> MHRVMGIETEYGISVPHQPNANAMAASSQVVNAYAPIGAPAQRQARWDFEEENPLRDARGFEVAREAADPSQLTDEDLGLANVILTNGARLYVDHAHPEYSTPEVTNPRDAVLWDKAGERIMAEAARRAADLPMGWTIQLYKNNTDNKGASYGCHENYLMNRSTPFADIVRHLIPFFVTRQVFCGAGRVGIGADGRGEGFQLSQRADFFEVEVGLETTLKRPIINTRDEPHADPEKYRRLHVIIGDANMSEIATYLKLGTTALVLAMIEDGFLSQDFSVESPVGALRAVSHDPTLRYQLRLHDGRRLTAVQLQMEYLEQARKYVEDRFGTDVDDMTRDVLDRWETTLVRLADDPMQLSRDLDWVAKLSILEGYRQRENLPWSAHKLQLVDLQYHDVRPDRGLYNRLVARGRMNLLVDEAAVRTAMHEPPNDTRAYFRGRCLAKFGAEIAAASWDSVIFDLPGRDSLQRVPTLEPLRGTRAHVGDLLDRCRSATELVAALTGGENLYFQ

Pupylation is the post-translational modification of lysine side chains with prokaryotic ubiquitin-like protein (Pup) that targets proteins for proteasomal degradation in mycobacteria and other members of Actinobacteria. A single Pup ligase enzyme, PafA (proteasome accessory factor A), is responsible for modifying all pupylation substrate proteins and likewise a single depupylase enzyme, Dop (deamidase of Pup), removes Pup from Pup-protein adducts. Depupylase Dop is structurally homologous to Pup ligase PafA, although the two evolutionarily related enzymes catalyze opposing reactions. Rather, before the catalytic cycle of Dop can begin, Dop-mediated cleavage of ATP in the active site must take place to generate the Pi species important for catalysis.

With the aim to capture Dop in a state where the Dop-loop could be resolved, crystallization experiments were carried out with AcelDop, exploring conditions with Dop alone and Dop in complex with Pup and/or different adenine nucleotides. We were successful in identifying crystallization conditions, where AcelDop in the absence of other ligands features the Dop-loop in a well-resolved conformation that is not induced via crystal contacts. In this structure, 33 of the 40 residues in the Dop-loop are resolved, including residues P40–R65 and L73–L80 and thereby all of the highly conserved residues in the loop. The Dop-loop features two very short helical stretches (DLη1 and DLα1) flanking a long zigzagging loop. Helix DLη1 (η stands for 310 helix) consists of residues 48-52 (DFEEE) and is located nearby the nucleotide-binding pocket (NBP) of Dop, while DLα1 is formed by residues 75-78 (DEDL) and is positioned distal to the active site. The Dop-loop forms extensive interactions with residues surrounding the active site. In particular, insertion of the highly conserved Dop-loop-residue W47 into the NBP leads to the formation of a triple π-stack, where W47 interacts with H231 that in turn stacks with W453 of the C-terminal domain. Another π-stacking interaction is formed by Dop-loop-residue F49 and H155. Furthermore, a network of salt bridges is formed between acidic residues in the Dop-loop and several arginine side chains surrounding the active site. Superimposition of the Dop-loop-inserted structure with any of the Pup-bound structures reveals dramatic conformational changes of the Dop-loop and several active site residues. The comparison shows that, upon binding of Pup, H95 swings upward by about 90° out of the way of Pup’s C-terminal residue and displaces the Dop-loop, including residue W47 that moves around 11 Å away from the NBP.> DMRPLNLAELNDCSRYPQTPNPTFAISPDIHPMPELTEPIQLKNHCAVFPTVALGESIYVYSHQIRKTPCKSEDTTHQRVSLGRIVDRGFSGPRASPLSTWDLQETEFLSSCSVAASGEIGWVLCVTTDKFTRDTVYAGPYTGLKLYKLSIRGQKEEYSITANNITTDAVIIALTLTRGSGVPKNNKLIFLGLAAVRDVDTTGVLCPTWKCDNINNNVGSCVHSYRLTADMNNYFMNVVVAVDVTPTGKMTASVSLLPMSESYIGSEGGVIDKPGGYGLMISNKGWFARIRYGQTDRASPQRYEWTDYMSFETPYYLYCSGGRICPVSCKTWNFTVPTILNPSGSIIIGVKAKSKTGNSASMITINTPDEVIDQYEVFNDYQSIGSTITKCFSYKRQPWCLVLLEGVLKSTGVTETSIQTFKIFRSCVKHRTYLDSLGTRFYYTVSDNGNKTKQTYIPGSDTGSGHHHHHHHH

Henipaviruses, a genus within the Paramyxoviridae family, include the highly virulent Nipah and Hendra viruses that cause reoccurring outbreaks of deadly disease. Recent discoveries of several new Paramyxoviridae species, including the zoonotic Langya virus, have revealed much higher antigenic diversity than currently characterized and prompted the reorganization of these viruses into the Henipavirus and Parahenipavirus genera. Here, to explore the limits of structural and antigenic variation in both genera, collectively referred to here as HNVs, we constructed an expanded, antigenically diverse panel of HNV fusion and attachment glycoproteins from 56 unique HNV strains that better reflects global HNV diversity. We expressed and purified the fusion protein ectodomains and the attachment protein head domains and characterized their biochemical, biophysical and structural properties.

A crystal structure of the Gamak virus attachment head domain revealed an additional domain added to the conserved 6-bladed, β-propeller fold.> KQFTKCELS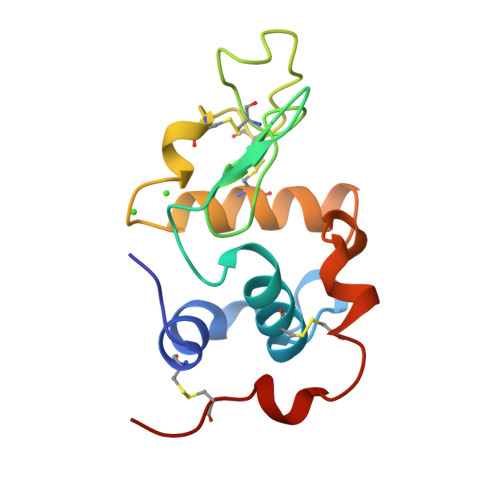QLLKDIDGYGGIALPELICTMFHTSGYDTQAIVENNESTEYGLFQISNKLWCKSSQVPQSRNICDISCDKFLDDDITDDIMCAKKILDIKGIDYWLAHKALCTEKLEQWLCEKL>GAMSPPAAPITLWTGPGPSINGFINDTPVIRCFICLTRDSNLVTVNASFVGEGGYRIVSPTQSQFSLIMEFDQFGQLMSTGNINST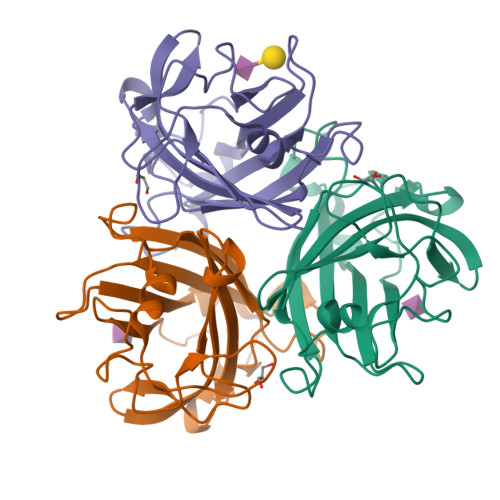TTWGEKPWGNNTVQPRPSHTWKLCMPNREVYSTPAATISRCGLDSIAVDGAPSRSIDCMLIINKPKGVATYTLTFRFLNFNRLSGGTLFKTDVLTFTYVGENQ[6x]> GAMGMKSRYTTEFHELEKIGSGEFGSVFKCVKRLDGCIYAIKRSKKPLAGSVDEQNALREVYAHAVLGQHSHVVRYFSAWAEDDHMLIQNEYCNGGSLADAISENYRIMSYFKEAELKDLLLQVGRGLRYIHSMSLVHMDIKPSNIFISRTSIPNAASEEGDEDDWASNKVMFKIGDLGHVTRISSPQVEEGDSRFLANEVLQENYTHLPKADIFALALTVVCAAGAEPLPRNGDQWHEIRQGRLPRIPQVLSQEFTELLKVMIHPDPERRP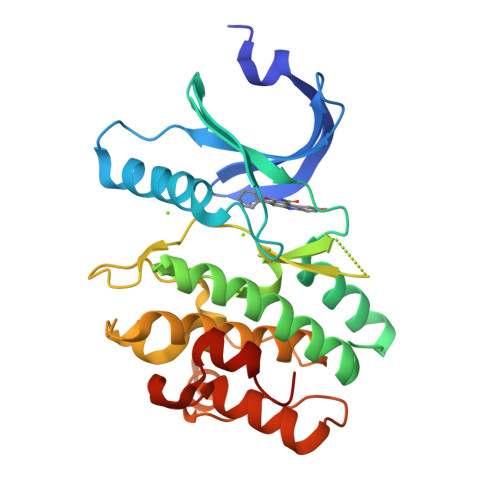SAMALVKHSVLLSASRK> MVKLNCRPLCQAPTASRLVSPPCFICRGVAPSA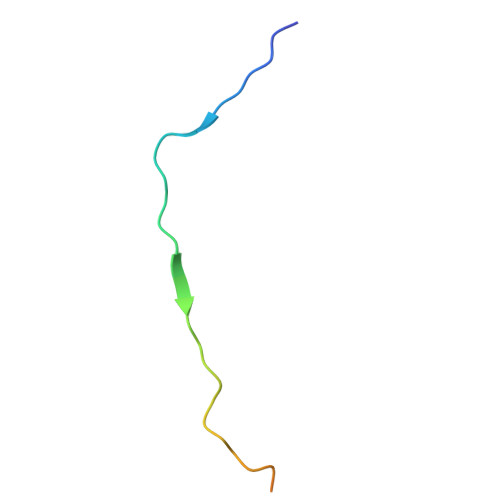PVTPG> MLEGKVKWFNSEKGFGFIEVEGQDDVFVHFSAIQGEGFKTLEEGQKVRFEIVEGNRGPQAANVT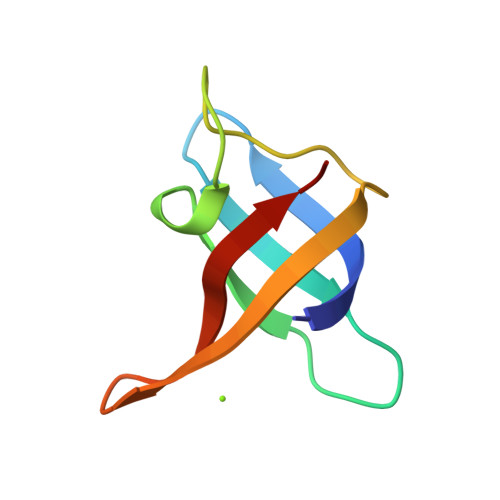KEA> GMQHHKVAIIGAGAAGIGMAITLKDFGITDVIILEKGTVGHSFKHWPKSTRTITPSFTSNGFGMPDMNAISMDTSPAFTFNEEHISGETY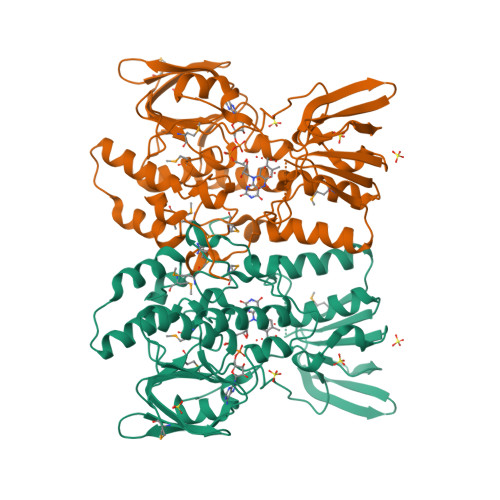AEYLQVVANHYELNIFENTVVTNISADDAYYTIATTTETYHADYIFVATGDYNFPKKPFKYGIHYSEIEDFDNFNKGQYVVIGGNESGFDAAYQLAKNGSDIALYTSTTGLNDPDADPSVRLSPYTRQRLGNVIKQGARIEMNVHYTVKDIDFNNGQYHISFDSGQSVHTPHEPILATGFDATKNPIVQQLFVTTNQDIKLTTHDESTRYPNIFMIGATVENDNAKLCYIYKFRARFAVLAHLLTQREGLPAKQEVIENYQKNQMYLDDYSCCEVSCTC> GAMGSIKEIAITHHVKEGHEKADPSQFELLKVLGQGSFGKVFLVKKISGSDARQLYAMKVLKKATLKVRDRVRTKMERDILVEVNHPFIVKLHYAFQTEGKLYLIL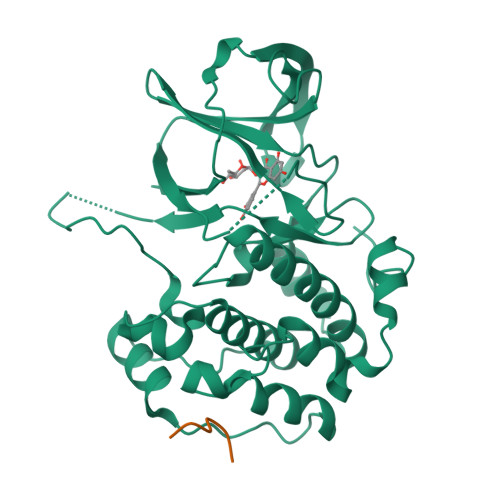DFLRGGDLFTRLSKEVMFTEEDVKFYLAELALALDHLHSLGIIYRDLKPENILLDEEGHIKLTDFGLSKESIDHEKKAYSFCGTVEYMAPEVVNRRGHTQSADWWSFGVLMFEMLTGTLPFQGKDRKETMTMILKAKLGMPQFLSPEAQSLLRMLFKRNPANRLGAGPDGVEEIKRHSFFSTIDWNKLYRREIHPPFKP;> STIHNEAELGDDDVFTTATDSSSNSSQKRE7-[[4-[(dimethylamino)methyl]phenoxy]methyl]quinolin-2-amine 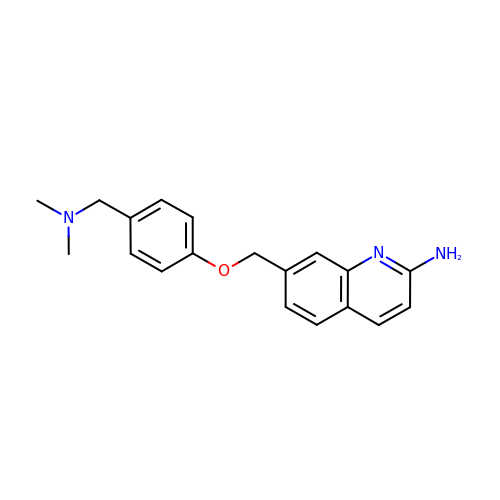| C19 H21 N3 O | RSUBEKFHYBPGDT-UHFFFAOYSA-N FlgA is a periplasmic flagellar protein that chaperones P-ring formation. FlgA possesses a typical signal sequence at its N-terminus, recognized by the Sec-dependent pathway, suggesting that FlgA functions as a P-ring assembly chaperone in the periplasm. P-ring formation is a key step enabling the bacterial flagellum to pass through the outer membrane. FlgA can be divided into three domains, denominated as D1 (residues 1–74), D2 (residues 75–142), and D3 (residues 143–198).

To gain insight into the regulatory mechanism of P-ring assembly by FlgA, two different atomic structures of FlgA from S. enterica, the open and closed forms were solved. Atomic models were built from amino acid residues Q1 through L198 (numbering corresponds to the mature protein) for the open and closed forms and refined at resolutions of 1.95 Å and 2.3 Å, respectively. For the open form, a segment from T44 thorough A47 was not traced in the final model due to the poor quality of the electron density map in this region. The conformation of FlgA is different in the two forms. While the structures of corresponding domains are similar in the open and closed forms, the D1 domains of the two forms align with an RMSD of 0.64 Å, while the D2 and D3 domains align with RMSDs of 0.35 Å and 0.33 Å, respectively. Based upon the structural difference induced by crystal packing, we tested whether the closed and open forms were possible in solution. FlgAR113C-S190C is locked in one conformation, while FlgA adopts intermediate structures upon immobilization, suggesting that FlgA might exist in the periplasm as a flexible intermediate structure, or in equilibrium between the open and closed forms defined here. Perhaps FlgA switches conformations from the closed to the open form after interacting with cellular components or other flagellar proteins.

> QDINAQLTTWFSQRLAGFSDEVVVTLRSSPNLLPSCEQPAFSMTGSAKLWGNVNVVARCANEKRYLQVNVQATGNYVAVAAPIARGGKLTPANVTLKRGRLDQLPPRTVLDIRQIQDAVSLRDLAPGQPVQLTMIRQAWRVKAGQRVQVIANGEGFSVNAEGQAMNNAAVAQNARVRMTSGQIVSGTVDSDGNILINLDPNSSSVDKLAAALEHHHHHH> MSDNLVLPTYDDVASASERIKKFANKTPVLTSSTVNKEFVAEVFFKCENFQKMGAFKFRGALNALSQLNEAQRKAGVLTFSSGNHAQAIALSAKILGIPAKIIMPLDAPEAKVAATKGYGGQVIMYDRYKDDREKMAKEISEREGLTIIPPYDHPHVLAGQGTAAKELFEEVGPLDALFVCLGGGGLLSGSALAARHFAPNCEV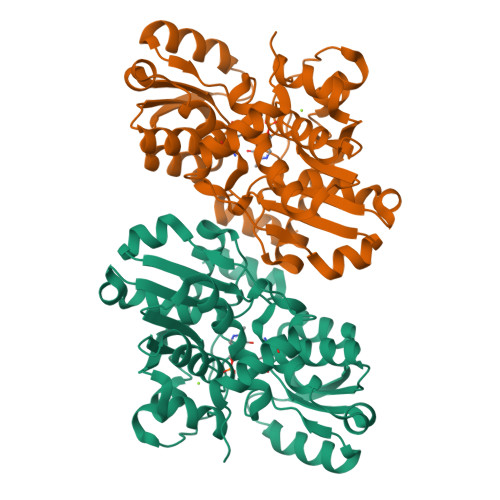YGVEPEAGNDGQQSFRKGSIVHIDTPKTIADGAQTQHLGNYTFSIIKEKVDDILTVSDEELIDCLKFYAARMKIVVEPTGCLSFAAARAMKEKLKNKRIGIIISGGNVDIERYAHFLSQ> MTTPTMQSTSLLTEHLGYPPISLVDDIINAVNEIMYKCTNAMEKYLMQRNIIGKKDFSDEIKIGTAKLESLLENSVDKNFDKLELYVLRNILSIPSDLLEENRFRLLHHEKLVLTDSATR;> MSVDRYSGMEGTEHIRFQRLVQVCN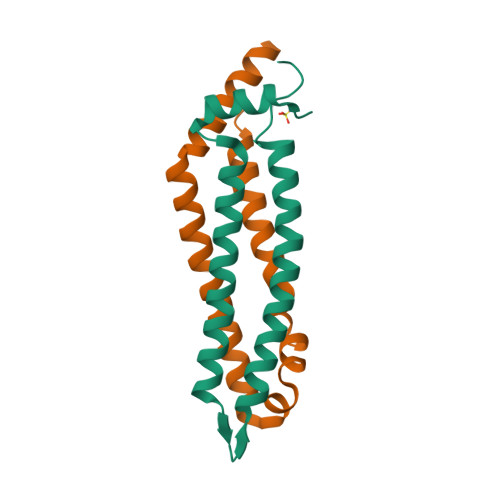KALEESIRKLQSWEKIHECFPNYGQTREGIENLTVCQQQVIKLWSNLSRVEFDAIFHERSIEEKLNQLDDLINKARS>GLTIDLKNFRKPGEKTFTQRSRLFVGNLPPDITEEEMRKLFEK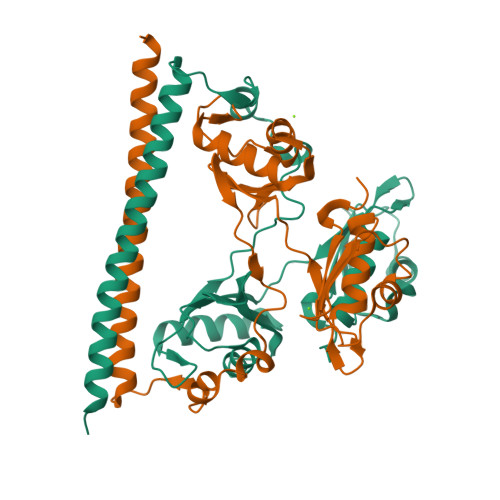YGKAGEVFIHKDKGFGFIRLETRTLAEIAKVELDNMPLRGKQLRVRFACHSASLTVRNLPQYVSNELLEEAFSVFGQVERAVVIVDDRGRPSGKGIVEFSGKPAARKALDRCSEGSFLLTTFPRPVTVEPMDQLDDEEGLPEKLVIKNQQFHKEREQPPRFAQPGSFEYEYAMRWKALIEMEKQQQDQVDRNIKEAREKLEMEMEAARHEHQVMLM[6x];>[6x]GFKANLSLLRRPGEKTYTQRCRLFVGNLPADITEDEFKRLFAKYGEPGEVFINKGKGFGFIKLESRALAEIAKAELDDTPMRGRQLRVRFATHAAALSVRNLSPYVSNELLEEAFSQFGPIERAVVIVDDRGRSTGKGIVEFASKPAARKAFERCSEGVFLLTTTPRPVIVEPLEQLDDEDGLPEKLAQKNPMYQKERETPPRFAQHGTFEYEYSQRWKSLDEMEKQQREQVEKNMKDAKDKLESEMEDAYHEHQANLL>[6x]MRPEPTEHPERTAAQRLYQYNVDLKVAFVLYAVAKLHLPDLLADGPRTTADLAAATGSDPSRLRRLLRAAAGADALREVPEDSFELAPMGDLLRSGHPRSMRGMTTFFAEPDVLAAYGDLVESVRTGVPAFQLRHREPLYDFLARPQHKEVRDEFDAAMVEFGQYFADDFLTSFDFGRFTRFADIGGGRGQFLAGVLTAVPSSTGVLVDGPAVAASAHKFLASQNLTERVEVRIG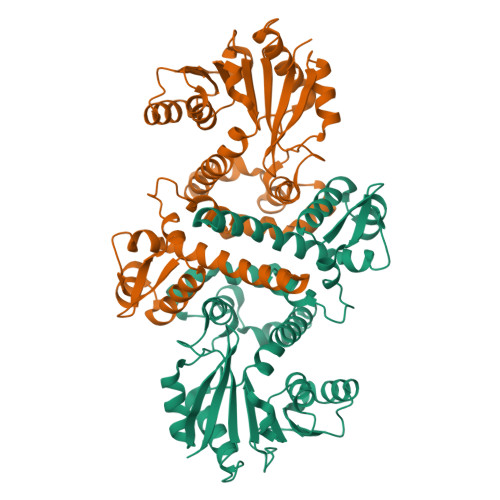DFFDVLPTGCDAYVLRGVLEDWADADAVRLLVRIRQAMGDAPEARLLILDSVIGETGELGKVLDLDMLVLVEGEHRTRAQWDDLLARAGFDIVGIHPAGDVWAVIECRGTAGHHHHHH>[2x]MELALGCSPAAQNGDTVPLPAVVPAPAAIEQATGAPFRLDASTRIEGEADAASALSALLEARTGLAPATGGDGAVIALRIEGGGPAESYALTADEASVTVTGADAAGLFYGVQTLGQLLARDGDAWVVPAVSIEDAPRFAYRGVMLDVARHFHPVETVKAYIGHAASLKLNALHLHLSDDQGWRIELHSRPELTALASSTAVGGDPGGFYTKDDYREIVEYAASRHMIVVPEIDMPSHTHAIGLAYPELAEEPVITDPMRETAAATGGALPESGTPYLGIEVGFSSLKIHDEATYDFAADVFGELAGMTPGPYLHLGGDEAHGTAEEDFALFVSRVSTIIADLGKTPVAWHEAGDAGGLAGATVGQYWGYVTPTDGMDDRARGFVSNGGQLILSPADAIYLDMKYPTGPDLG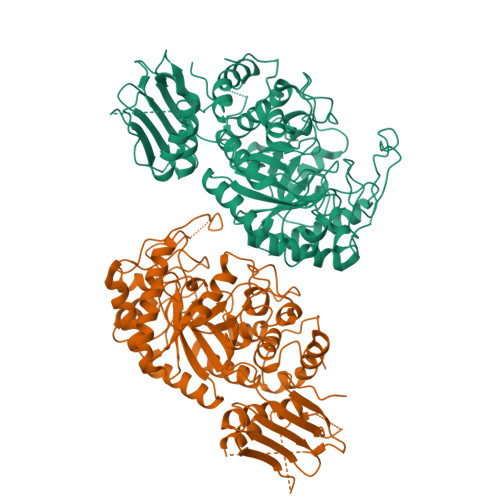LSWANGPTSVQRAYDWEPSTVIPGIDDADILGVEAPLWSETLRSLDDIETMAFPRIAAAAEAAWSPATGASDLRTWESFRARVGALGPLWTSLGIGFHPSGEIDWATEKGQFLEHHHHHH> MKPTMAILERISKNSQENIDEVFTRLYRYLLRPDIYYVAYQNLYSNKGASTKGILDDTADGFSEEKIKKIIQSLKDGTYYPQPVRRMYIAKKNSKKMRPLGIPTFTDKLIQEAVRIILESIYEPVFEDVSHGFRPQRSCHTALKTIKREFGGARWFVEGDIKGC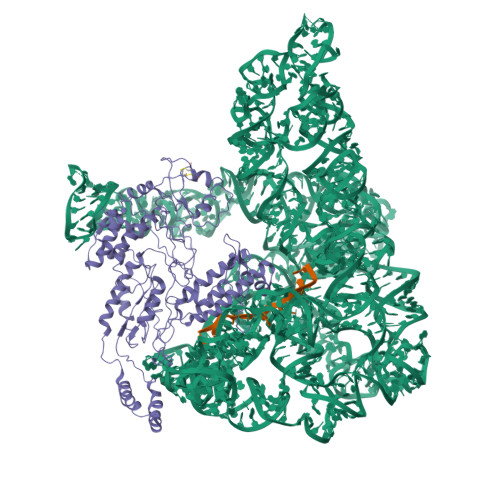FDNIDHVTLIGLINLKIKDMKMSQLIYKFLKAGYLENWQYHKTYSGTPQGGILSPLLANIYLHELDKFVLQLKMKFDRESPERITPEYRELHNEIKRISHRLKKLEGEEKAKVLLEYQEKRKRLPTLPCTSQTNKVLKYVRYADDFIISVKGSKEDCQWIKEQLKLFIHNKLKMELSEEKTLITHSSQPARFLGYDIRVRRSGTIKRSGKVKKRTLNGSVELLIPLQDKIRQFIFDKKIAIQKKDSSWFPVHRKYLIRSTDLEIITIYNSELRGICNYYGLASNFNQLNYFAYLMEYSCLKTIASKHKGTLSKTISMFKDGSGSWGIPYEIKQGKQRRYFANFSECKSPYQFTDEISQAPVLYGYARNTLENRLKAKCCELCGTSDENTSYEIHHVNKVKNLKGKEKWEMAMIAKQRKTLVVCFHCHRHVIHKHK>ALHKGSAAAPALQKDSKKRVFSGIQPTGILHLGNYLGAIESWVRLQDEYDSVLYSIVDLHSITVPQDPAVLRQSILDMTAVLLACGINPEKSILFQQSQVSEHTQLSWILSCMVRLPRLQHLHQWKAKTTKQKHDGTVGLLTYPVLQAADILLYKSTHVPVGEDQVQHMELVQDLAQGFNKKYGEFFPVPESILTSMKKVKSLRDPSAKMSKSDPDKLATVRITDSPEEIVQKFRKAVTDFTSEVTYDPAGRAGVSNIVAVHAAVTGLSVEEVVRRSAGMNTARYKLAVA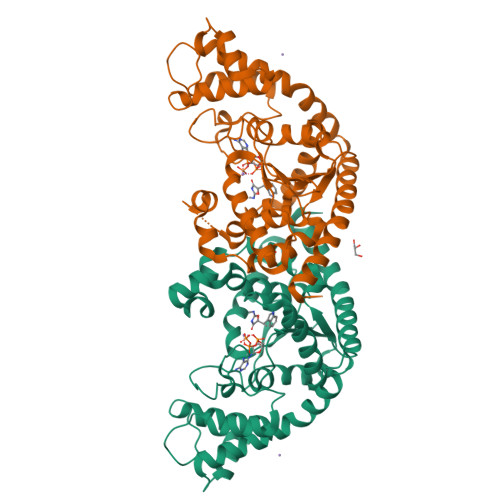DAVIEKFAPIKREIEKLKLDKDHLEKVLQIGSAKAKELAYTVCQEVKKLVGFL[2x]>[2x]MSGRDISTAVVVTTISDGGFLDRLAPALRDAGARLIVIPDRNTGPALFAACERHRRLGLDVVCPSVAEQQDLLERLAVPDLIPYHSDNRRNVGYLMAWMEGFDVIVSMDDDNLPTTDDFVERHQVVCQGPRTQPVTASSDGWFNNCALLEVEPTEVFPRGFPFHARPAHAQARTSVCERPADVRINAGLWLGDPDVDAITRLAVRPNALAHSGGSVVLAEGTWCPVNSQN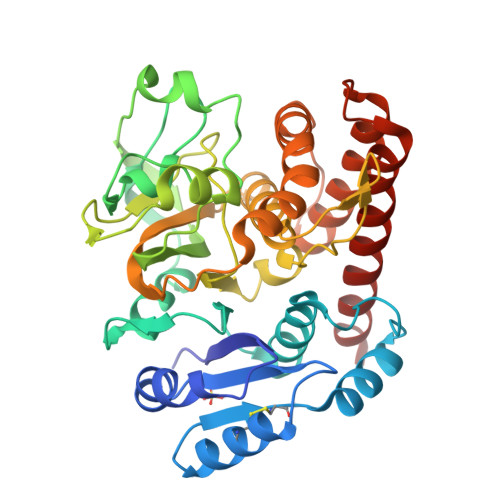TAVHRDALPAYYFLRMGQPVDGVPMERFGDIFSGYFVQVCAQHLGHAVRFGDPVVEHPRNEHDLLDDLHKEVPAVRLLDDILDHLRDHPLEGGDYLETYESLSYALQEIAERVNGRAWSPDARAFLHRSAHLMRSWTGALRTVAGT> MASETPRVDPTEISNVNAPVFRIIAQIKSQPTESQLILQSPTISSKNGSEVEMITLNNIRVSMNKTFEIDSWYEFVCRNNDDGELGFLILDAVLCKFKENEDLSLNGVVALQRLCKKYPEIY;> TNTRVNTLTPVTIKQILESKQDIQDGPFVSHNQELHHVCFVGVVRNITDHTANIFLTIEDGTGQIEVRKWSEDAAQQFEIGGYVKVFGALKEFGGKKNIQYAVIKPIDSFNEVLTHHLEVIKCHSIASGMMK;> KFIAQRITIARAQAENLGRSEKGDFFSVKAAISFLKVDNFAYPACSNENCNKKVLEQPDGTWRCEKCDTNNARPNWRYILTISIIDETNQLWLTLFDDQAKQLLGVDANTLMSLKEE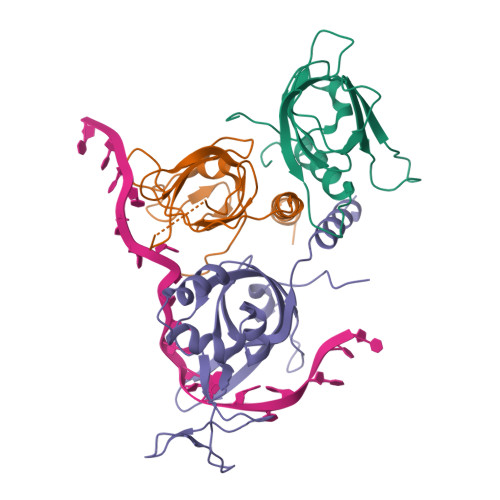DPNEFTKITQSIQMNEYDFRIRAREDTYNDQSRIRYTVANLHSLNYRAEADYLADELSKAL> MASSPQRGRPRLNAARTTFVGDNGQPLRGPYTSTEWTAAAPYDQIARVKELGFNAVHLYAECFDPRYPAPGSKAPGYAVNEIDKIVERTRELGLYLVITIGNGANNGNHNAQWARDFWKFYAPRYAKETHVLYEIHNEPVAWGPPYSSSTANPPGAVDMEIDVYRIIRTYAPETPVLLFSYAVFGGKGGAAEALKDIRAFNKAVFGNENAVWTNEAVAFHGYAGWQETTIAVEELLKAGYPCFMTEYAGGAWGSGMGGLDVELTYELERLGVSWLTFQYIPPTGVSDDVTKPEYFSALVENSGLSWTPDYGNWPAARGVYGNGGLARETATWINNFLTGTTRIEAEDFDWGGNGVSYYDTDSVNVGGQYRPDEGVDIEKTSDTGGGYNVGWISEGEWLEYTIRVRNPGYYNLSLRVAGISGSRVQVSFGNQDKTGVWELPATGGFQTWTTATRQVFLGAGLQKLRINALSGGFNLNWIELSPILE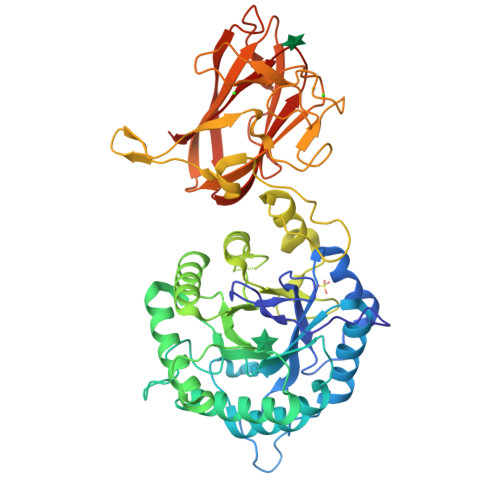HHHHHH A further enzyme, McbA, has recently been reported in the biosynthetic pathway towards the marinacarbolines in Marinactinospora thermotolerans by Ji and co‐workers. McbA catalyzes the ATP‐dependent coupling of the β‐carboline derivative 6 with 2‐phenylethylamine a to form 6 a via adenylate 7, but, unlike other ABSs, McbA also accepted other amines, including substituted 2‐phenylethylamines and tryptamines, thus indicating some promise for the application of this enzyme to reactions with a wider substrate spectrum. McbA adopts a structure within the ANL superfamily of adenylating enzymes defined by Gulick, and which includes firefly luciferase, acetyl‐CoA synthase, and standalone adenylation domains of NRPSs, including the dihydroxybenzoate adenylating enzyme enzyme DhbE20 from the bacillibactin biosynthetic pathway. Each ANL enzyme is characterized by a two‐domain structure in which a large N‐terminal domain is coupled to a smaller C‐terminal one, consisting of 4–500 and 100 amino acid residues, respectively.

To investigate the promiscuity in term of aryl acid recognition by McbA, the structure of the enzyme was determined using X‐ray crystallography. A K483A mutant co‐crystallised with AMP, magnesium ions, and the β‐carboline acid substrate 6 yielded crystals of diffraction quality. The structure was solved using molecular replacement, and refined to a resolution of 2.80 Å (data collection and refinement statistics can be found in Table S2 in the Supporting Information). The McbA structure features the two predicted domains: the large N‐terminal domain of residues 1–394 (McbAN) and the smaller C‐terminal one comprising residues 395–494 (McbAC), with the hinge residue at Q394. Crucially, the structures of many ANL enzymes have revealed substantial relative domain rotation during the reaction coordinate, with one conformation (“adenylation”) assumed for adenylate formation from the carboxylate substrate and ATP, and a second, (“thiolation”) in which the C‐terminal domain rotates to enable the ligation reaction between the phosphopantetheinate thiol and the adenylate intermediate. The substrate 6 is bound within a hydrophobic pocket stacked between the loop between G295 and F301 on one face and L202 on the other. Few specific interactions between active‐site residues and the substrate are made, except that the carbonyl oxygen and pyridine nitrogen of 6 interact with the backbone N‐H and C=O of G295 at distances of approximately 3.9 and 3.4 Å respectively. The relative lack of specific interactions may help to explain the relaxed specificity of McbA for the range of aryl acids used in this study. The exception was quinoline derivative 18, in which the N‐atom in the 1‐position has had an adverse effect on conversion, perhaps disrupting the hydrophobic interaction made by the native ligand with F301.

>QGPAMGYARRVMDGIGEVAVTGAGGSVTGARLRHQVRLLAHALTEAGIPPGRGVACLHANTWRAIALRLAVQAIGCHYVGLRPTAAVTEQARAIAAADSAALVFEPSVEARAADLLERVSVPVVLSLGPTSRGRDILAASVPEGTPLRYREHPEGIAVVAFTSGTTGTPKGVAHSSTAMSACVDAAVSMYGRGPWRFLIPIPLSDLGGELAQCTLATGGTVVLLEEFQPDAVLEAIERERATHVFLAPNWLYQLAEHPALPRSDLSSLRRVVYGGAPAVPSRVAAARERMGAVLMQNYGTQEAAFIAALTPDDHARRELLTAVGRPLPHVEVEIRDDSGGTLPRGAVGEVWVRSPMTMSGYWRDPERTAQVLSGGWLRTGDVGTFDEDGHLHLTDRLQDIIIVEAYNVYSRRVEHVLTEHPDVRAAAVVGVPDPDSGEAVCAAVVVADGADPDPEHLRALVRDHLGDLHVPRRVEFVRSIPVTPAGAPDKVKVRTWFTD[5x]>NAIAVVVDKEPITTYDIDQTMKALKIDRNKALGVLINEKMEISQMKQLGIVVNDLELDDAINKMLAQNKTTLNAFKANLKSKNQSYEQFRTNFKKDLEKRKLYEKIASMAKTDFSDDGAKKFFEQNKDKFTFYTQINANIYLSNNPQTLENIKNTKKTILKPQNASLNTSNADPRLLGLLSQIPVGSFSPVLNGKNGYELYEVKSKDGT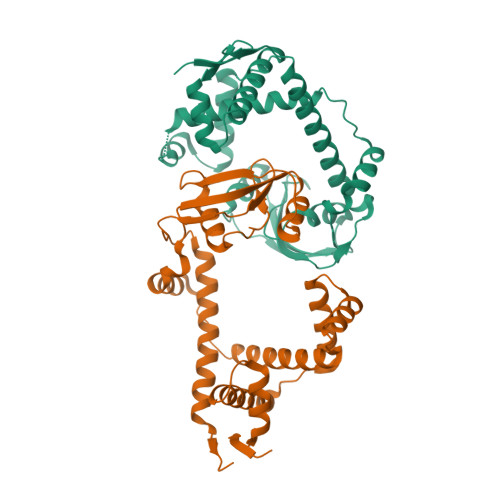QTPEYEQVKNEVLNAYVSEQRQNFIQDYFDKLRSKINIEYLRA[2x]>LPISMSDEGDSFLVKDSLGENKIPKNPSKVVILDLGILDTFDALKLNDKVVGVPAKNLPKYLQQFKNKPSVGGVQQVDFEAINALKPDLIIISGRQSKFYDKLKEIAPTLFVGLDNANFLSSFENNVLSVAKLYGLEKEALEKISDIKNEIEKAKSIVDEDKKALIILTNSNKISAFGPQSRFGIIHDVLGINAVDENIKVGTHGKSINSEFILEKNPDYIFVVDRNVILGNKERAQGILDNALVAKTKAAQNKKIIYLDPEYWYLASGNGLES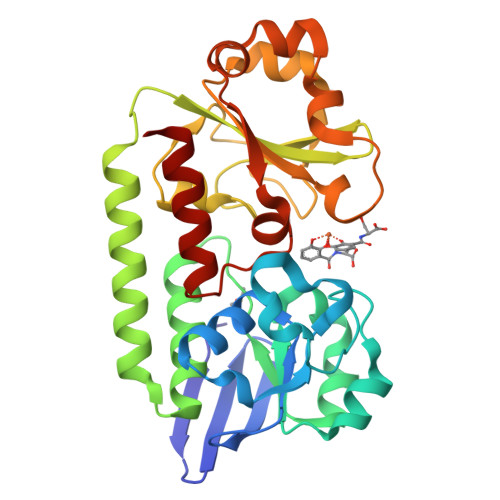LKTMILEIKNAVK[3x]In this study, we report a detailed characterization of ΦCjT23, an icosahedral temperate ssDNA phage with an inner lipid membrane, isolated earlier from a strain of Flavobacterium (previously Cytophaga). The virion structure determined by cryogenic electron microscopy reveals similarities to members of the viral kingdom Bamfordvirae that currently consists solely of dsDNA viruses with a major capsid protein composed of two upright β-sandwiches. The minimalistic structure of ΦCjT23 suggests that this phage serves as a model for the last common ancestor between ssDNA and dsDNA viruses in the Bamfordvirae. Both ΦCjT23 and the related phage FLiP infect Flavobacterium species found in several environments, suggesting that these types of viruses have a global distribution and a shared evolutionary origin.

To address distant evolutionary relationships, we determined the structure of the ΦCjT23 virion by cryo-EM. Single-particle analysis of complete particles resulted in an icosahedrally symmetric reconstruction with an average estimated resolution of 4.1 Å. The observed 200 MCP trimers, occupying four unique positions in the asymmetric unit, follow icosahedral capsid organization characterized by a pseudo-triangulation number T = 21. Within the asymmetric unit, type 1 trimers circle the five-fold symmetry axes at the vertices, type 2 trimers reside on both sides of the icosahedral two-fold axis of symmetry, type 3 trimers reside on the icosahedral three-fold axis of symmetry (contributing one MCP per asymmetric unit) and type 4 trimers reside between the rest. The asymmetric unit contains 10 independent MCP monomers, contributing a total of 20 β-sandwiches (V1 and V2). The penton domain of the spike presents one monomer per asymmetric unit and constitutes an additional building block. As these 21 building blocks are not identical in sequence (MCP V1, MCP V2, and penton domain of the spike protein), the triangulation is referred to as ‘pseudo’. The dimensions of the faceted capsid are characterized by a face-to-face distance of ~55 nm, an edge-to-edge distance of ~54 nm, and a vertex-to-vertex distance of ~63 nm. Inside, a lipid bilayer with a thickness of ~5 nm is discernible. Spike proteins extend from the 12 vertices, but the density corresponding to these was disordered in the icosahedrally averaged map due to the presence of a flexible hinge region in the spike.

>MKIATITGVTKSPELQVTKAIGALILSSDVALSALTTEKISIYIERGNGSNVILANKVLLKDFILASTYGTENTQSDADNAMIALCELADEGSIYLADKESIKITLEDLISDKRYDLHGIEEPQQTNNLFFFEQKSVASEEFNKKIDVQGFDLAIMTVDDSVSDLSYQYSNGQVVKYLPFELQTLSRDIDPIQAVLSDGKVVQGLTDRLTLPLVAVVGIEINKSQGSIINFVVRCLKTV[10x];> MNFIQYIDDSYAVKVKEINSSEGFYINGIQTPFFILSVFIGNKRVTGVEFNNYDSLPMLSVINDLGNIDLNVIPQNYFATAFTEIYFNIPF>MNTINIAKNDFSDIELAAIPFNTLADHYGERLAREQLALEHESYEMGEARFRKMFERQLKAGEVADNAAAKPLITTLLPKMIARINDWFEEVKAKRGKRPTAFQFLQEIKPEAVAYITIKTTLACLTSADNTTVQAVASAIGRAIEDEARFGRIRDLEAKHFKKNVEEQLNKRVGHVYKKAFMQVVEADMLSKGLLGGEAWSSWHKEDSIHVGVRCIEMLIESTGMVSLHRQNAGVVGQDSETIELAPEYAEAIATRAGALAGISPMFQPCVVPPKPWTGITGGGYWANGRRPLALVRTHSKKALMRYEDVYMPEVYKAINIAQNTAWKINKKVLAVANVITKWKHCPVEDIPAIEREELPMKPEDIDMNPEALTAWKRAAAAVYRKDKARKSRRISLEFMLEQANKFANHKAIWFPYNMDWRGRVYAVSMFNPQGNDMTKGLLTLAKGKPIGKEGYYWLKIHGANCAGVDKVPFPERIKFIEENHENIMACAKSPLENTWWAEQDSPFCFLAFCFEYAGVQHHGLSYNCSLPLAFDGSCSGIQHFSAMLRDEVGGRAVNLLPSETVQDIYGIVAKKVNEILQADAINGTDNEVVTVTDENTGEISEKVKLGTKALAGQWLAYGVTRSVTKRSVMTLAYGSKEFGFRQQVLEDTIQPAIDSGKGLMFTQPNQAAGYMAKLIWESVSVTVVAAVEAMNWLKSAAKLLAAEVKDKKTGEILRKRCAVHWVTPDGFPVWQEYKKPIQTRLNLMFL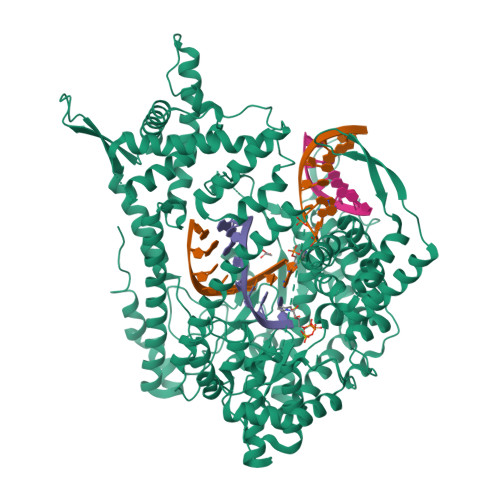GQFRLQPTINTNKDSEIDAHKQESGIAPNFVHSQDGSHLRKTVVWAHEKYGIESFALIHDSFGTIPADAANLFKAVRETMVDTYESCDVLADFYDQFADQLHESQLDKMPALPAKGNLNLRDILESDFAFA[4x]> IQITRGDSTITSQDTANAV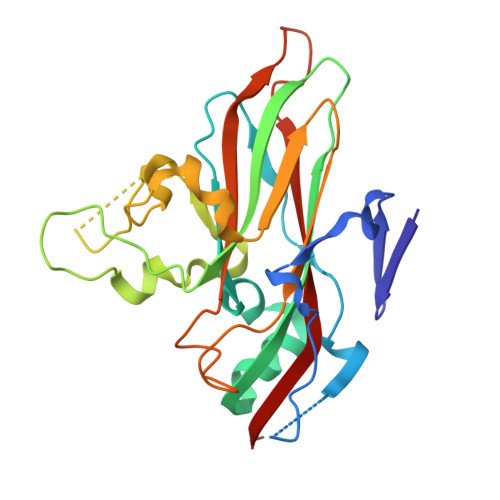VAYGVWPSYLTPDDATAIDKPTQPDTSSNRFYTLDSRSWTSASSGWWWKLPDALKNMGIFGENMFYHFLGRSGYTIHVQCNSSKFHQGLLIVAAIPEHQLASATSGNVSVGYNHTHPGEQGREVVPSRTSSDNKRPSDDSWLNFDGTLLGNLPIYPHQYINLRTNNSATLILPYVNAVPMDSMLRHNNWSLVIIPICPLQVQPGGTQSIPITVSISPMFSEFSGPRS> VVGGTRAAQGEFPFMVRLSMGCGGALYAQDIVLTAAHCVSGSGNNTSITATGGVVDLQSSSAVKVRSTKVLQAPGYNGTGKDWALIKLAQPINQPTLKIATTTAYNQGT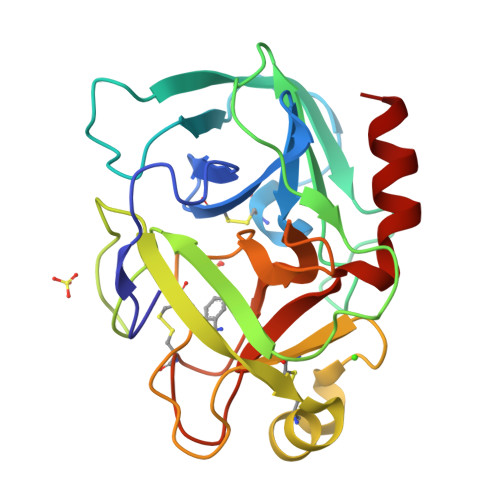FTVAGWGANREGGSQQRYLLKANVPFVSDAACRSAYGNELVANEEICAGYPDTGGVDPCQGDSGGPMFRKDNADEWIQVGIVSWGYGCARPGYPGVYTEVSTFASAIASAARTL> ETDEEPEEPGRRGSFVEMVDNLRGKSGQGYYVEMTVGSPPQTLNILVDTGSSNFAVGAAPHPFLHRYYQRQLSSTYRDLRKGVYVPYTQGKWEGELGTDLVSIPHGPNVTVRANIAAITESDKFFINGSNWEGILGLAYAEIARPDDSLEPFFDSLVKQTHVPNLFSLQLCGAGF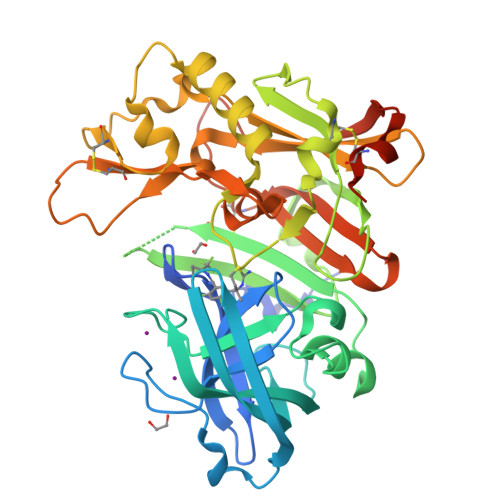PLNQSEVLASVGGSMIIGGIDHSLYTGSLWYTPIRREWYYEVIIVRVEINGQDLKMDCKEYNYDKSIVDSGTTNLRLPKKVFEAAVKSIKAASSTEKFPDGFWLGEQLVCWQAGTTPWNIFPVISLYLMGEVTNQSFRITILPQQYLRPVEDVATSQDDCYKFAISQSSTGTVMGAVIMEGFYVVFDRARKRIGFAVSACHVHDEFRTAAVEGPFVTLDMEDCGYNIPQTDESTHHHHHH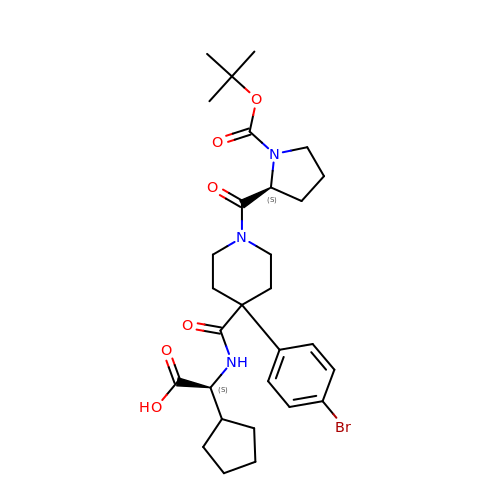(2S)-({4-(4-bromophenyl)-1-[1-(tert-butoxycarbonyl)-L-prolyl]piperidine-4-carbonyl}amino)(cyclopentyl)acetic acid | C29 H40 Br N3 O6 | CZJLHKGARYEGAY-GOTSBHOMSA-N>MELTDEEASFLTRRQLLALSENGDLPDDIEYEVDLDLKFANNRLKRAYIALQAWKKAFYSDPFNTAANWVGPDVCSYKGVFCAPALDDPSVLVVAGIDLNHADIFGYLPPELGLLTDVALFHVNSNRFCGVIPKSLSKLTLMYEFDVSNNRFVGPFPTVALSWPSLKFLDIRYNDFEGKLPPEIFDKDLDAIFLNNNRFESTIPETIGKSTASVVTFAHNKFSGCIPKTIGQMKNLNEIVFIGNNLSGCLPNEIGSLNNVTVFDASSNGFVGSLPSTLSGLANVEQMDFSYNKFTGF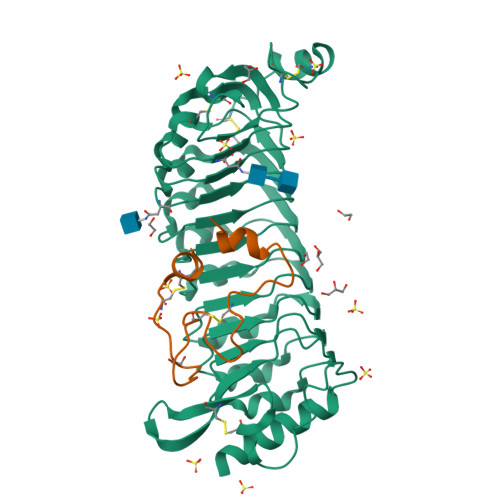VTDNICKLPKLSNFTFSYNFFNGEAQSCVPGSSQEKQFDDTSNCLQNRPNQKSAKECLPVVSRPVDCSKDKCAGG[2x];>[2x]ARGRRYIGYDALKKNNVPCSRRGRSYYDCKKRRRNNPYRRGCSAITHCYR TMEM95 is a type I single-pass transmembrane protein. Tmem95 encodes a sperm acrosomal membrane protein, which relocalizes to the equatorial segment of the sperm head where membrane fusion with the egg takes place. Tmem95 knockout murine sperm, which have normal expression and localization of IZUMO1, can bind to, but do not fuse with, eggs. We propose that the interaction of TMEM95 with eggs facilitates membrane fusion of human sperm and eggs.

To understand how TMEM95 binds eggs, we determined a crystal structure of the TMEM95 ectodomain to 1.5 Å resolution using multiwavelength anomalous X-ray diffraction. TMEM95 adopts an elongated rod shape, comprised of an N-terminal α-helical bundle (residues 17 to 110) and a C-terminal β-hairpin region (residues 111 to 135). The helical bundle of TMEM95 has three helices (α1, α3, and α4) and a coil (loop 2) that are arranged in an anti-parallel manner (α1-loop 2 and α3-α4). TMEM95 has three unique disulfide bonds: C35-C45 between α1 and loop 2, and C105-C134 and C109-C128 adjacent to the β-hairpin. TMEM95 shows homology to the N terminus of IZUMO1 (14, 15) with a Cα root-mean-square deviation of 7.2 Å and to the N terminus of SPACA6 (17). Unlike IZUMO1 and SPACA6, TMEM95 does not have an immunoglobulin-like domain at the C terminus. A conserved N-linked glycan in the β-hairpin of TMEM95 could cause a clash if TMEM95 were to make a contact similar to that of IZUMO1 with JUNO. We found that the area surrounding the N-glycan is variable, while the opposite side harbors a conserved, positively charged surface. When incubated with hamster eggs, the R70A, R73A, and R70A R73A TMEM95-Fc variants showed drastically reduced egg-binding activities compared to the wild-type. Our data suggest that the identified evolutionarily conserved, positively charged surface of TMEM95 may function as a receptor-binding site.

> CVFCRLPAHDLSGRLARLCSQMEARQKECGASPDFSAFALDEVSMNKVTEKTHRVLRVMEIKEAVSSLPSYWSWLRKTKLPEYTREALCPPACRGSTTLYNCSTCKGTEVSCWPRKRCFPGS Corticosteroid-binding globulin (CBG) is a glycosylated plasma protein implicated in steroid transport and delivery. By its primary structure, CBG is classified as a clade A member of the serine protease inhibitor (SERPIN) family, together with the closely related alpha-1-antichymotrypsin, alpha-1-antitrypsin (AAT) and thyroxine-binding globulin (TBG). Contrary to the proteinase inhibitors alpha-1-antichymotrypsin and AAT, CBG and TBG have no known inhibitory function. While CBG does not act as a protease inhibitor, it is a substrate for neutrophil elastase and becomes cleaved in the reactive center loop (RCL).

It represents the first crystal structure of CBG in complex with progesterone and, more importantly, the sequence of the RCL corresponds to that of wild-type CBG and is not replaced by the sequence of AAT Pittsburgh as in a previous study with a CBG-AAT chimera. Second, the RCL was cleaved during crystallization, and upon structure solution it became obvious that CBG is depicted in the SERPIN R-conformation with a fully antiparallel six-stranded β-sheet A, in which the RCL is integrated as β-strand s4 into sheet A. The RCL is cleaved after Thr349 or Ser350. If cleavage occurred after Thr349, the cleavage site would be homologous to that of human AAT after cleavage with neutrophil elastase. As a result of this novel cleavage site, the inserted RCL segment is four residues longer than expected, and a more extended β-strand s4 is formed with additional main-chain hydrogen bonds with neighboring strands s3 and s5. From a structural point of view, this novel cleavage site makes sense because it allows for the formation of an extended β-strand s4A with main-chain hydrogen-bonds connecting the former RCL segment to strands s5A and s3A over the entire length of β-sheet A. The stacking of the indol ring of Trp371 against the cyclohexane ring of progesterone constitutes a hallmark for ligand binding to CBG. Trp371 itself packs via a cation-π-interaction with Arg15. Only a single direct hydrogen bond is formed between progesterone and CBG, namely between the carbonyl oxygen at C-20 and the side chain of Gln232. Our structural data suggest that this difference can be attributed to the fact that progesterone does not form some of the hydrogen bonds observed in the cortisol complex because it lacks the hydroxyl groups attached to atoms C-11 and C-17.

> GSNHHRGLASANVDFAFSLYKHLVALSPKKNIFISPVSISMALAMLSLGTCGHTRAQLLQGLGFNLTERSETEIHQGFQHLHQLFAKSDTSLEMTMGNALFLDGSLELLESFSADIAHYYESEVLAMNFQDWATASRQINSYVKNKTQGKIVDLFSGLDSPAILVLVNYIFFKGTWTQPFDLASTREENFYVDETTVVKVPMMLQSSTISYLHDSELPCQLVQMNYVGNGTVFFILPDKGKMNTVIAALSRDTINRWSAGLTSSQVDLYIPKVTISGVYDLGDVLEEMGIADLFTNQANFSRITQDAQLKSSKVVHKAVLQLNEEGVDTAGSTGVTLNLT;> SKPIILRFNQPFIIMIFDHFTWSSLFLARVMNPV> DRKRRSDPNFKNRLRERRKKQKLAKERAGLSKLPDLKDAEAVQKFFLEEIQLGEELLAQGEYEKGVDHLTNAIAVCGQPQQLLQVLQQTLPPPVFQ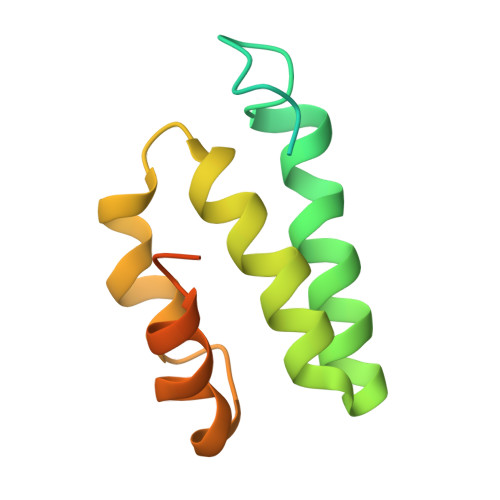MLLTKLPTISQRIVSAQSLAEDDVE>MRKFILSLSILLSALLVACSSRNHYGDTGSLAGLQAMADSKYTRAQKKQKMGKIREMALKETALSVGAQAGLAWRAKIIDEQLNKQARNLDAIYDFNSLVLEHNILPPVLLEGRNTLNLADAQSIRISDRTYKVAKQAHFITTPPTWRQYLWMDYVKPEAPNVTLLPKTKAEKEIWCIYTERGWKNGIDQANTILEENIARIKEDFGGMILYRKLLAMNMVSPPYVSHTDLGVTGDGSEIHIDDRVLRITALPELNVNSAEWRAAVAKDENALERFKNMEKLANQAKIVITNKSWQPIIAPVS[13x];>MNNNKIVIMFIFSALLAGCAGTMKFKKPPINNPSDDATIKLAEAAVSVSDSMLEMAKVEKVITPPSKDNTLTIPNAYNLQARASVDWSGPIEELTARIAKAAHFRFRVLGKSPSVPVLISISTKDESLAEILRDIDYQAGKKASIHVYPNSQVVELRYAKIYS[26x];>[31x]MMAEHDQNNDEYKFAELDSYDMDQAGESDLDSEASYQSGKEGLTKKKDIKRNALIAIGAVVFIMVMYKIIGWMFFSDKSSQVTSKPAIPPVTQVATPQPVQTIPTTTPIQQVQPTTIIEDDPDLKKKVSAIEMTQQSLRSEVNALSEQINAVNNNIKNLNAQIVNLNQIIGNMSNQIARQSEVINVLMARTTPKKVVKVSRPIVQARIIYYIQAVIPGRAWLIGSNGSTLTVREGSKIPGYGMVKLIDSLQGRILTSSGQVIKFSQEDS;>MASKKENLKSLFSNTRTRVIIIFTAALLIIAVVIGFFKIRGATTGSIAAAEVSTVPGGIQSIPGVLDPTAQYAKLQEEQNITQAQVAEKTGGSAIPTIIRTQALGEGVGVIGSQSGVGFAALAQEELGGPQRSLWIQELQDGSCSKSVITKVVNQGAQLTDLKAACSCVQLKDSGYGLQELEQVCECKELKSAGYNARQLKEAGYSAGRLRNCGFDACELRNAGFTAQEMKDGGFSDGELKGAGFSDAEIAKASGLPDGITADDVRKAGCGAAALAKLRQAGVSASAIRKISGCTAEQLKAAGYTAKELKDAGFSAADLRRAGFSAAELKDAGFTARDLLNAGFTPADLAKAGFSDAQIKAAQAELPPGITPQDVKNAGCDVEALKKEREAGVSAALIRQYAGCSAQALKAAGFTDADLANAGFTPAQISAATPLSDAEIKAAGCDPDKLKKLFSAGVSAKRIKELNGCSAEALKAAGYDAQSLLAAGFTPQELLAAGFTPKQLEDAGLNPVSIIADGRVADCSVESLKKARAAGVSALTIKQTLGCSAAALKAAGYTAKELKDAGFTAAELKAAGFSAKELKDAGFTAKELRDAGFSAQELKDVGFSAKDLKDAGFSAAELKAAGFTAAQLKAAGFSAKDLKDAGFSAAELKAAGFSAKELKDAGFSASDLKNAGFSAKELKDAGFSASDLKSAGFSASELKNAGYSADELKKAGYTSAELRNAGFSPQESAVAGLQGPDLQQLDSSITGIPSIPGATPRPTTSDAASSAEQLQAILQKQNEQLAEQKYQQEIQQRTSDMLTAATQLVQDWKQVETQVYTEGTEETKTSGGESAVPGTGTGTGSNNQPVDQGAVSAQNQAIIKTGDIMFAVLDTSVNSDEPGPILATIVTGKLKGSKLIGSFNLPSNADKMVITFNTMSIPGAEKTISISAYAIDPNTARTALASRTNHHYLMRYGSLFASSFLQGFGNAFQSANTTITIGGTGGGNNITVANGVGRSTLENAVIGLATVGKAWSQQAQQLFNTPTTVEVYSGTGLGILFTQDVTTI[18x];>[18x]MMKKYDQLCKYCLVIGLTFSMSCSIYAADQSDDAQQALQQLRMLQQKLSQNPSPDAQSGAGDGGDNAASDSTQQPNQSGQANAPAANQTATAGGDGQIISQDDAEVIDKKAFKDMTRNLYPLNPEQVVKLKQIYETSEYAKAATPGTPPKPTATSQFVNLSPGSTPPVIRLSQGFVSSLVFLDSTGAPWPIAAYDLGDPSSFNIQWDKTSNTLMIQATKLYNYGNLAVRLRGLNTPVMLTLIPGQKAVDYRVDLRVQGYGPNAKSMPTEEGIPPSANDLLLHVLEGVPPPGSRRLVVSGGDARAWLSNEKMYVRTNLTILSPGWLASMTSADGTHAYEMQKSPVLLVSWHGKVMQLKVEGL;>[13x]MRSLRTNYIYVLFKTTGLLFLLLLSACNRSGYIPENEVPKLPCRVDGACDATIIKMMTDLNKKGIKVASVGQNYLISIPASALFADQSPRLNWASYSLLNEIAAFLKQFRKIAITVTSYSSKYVSVKRERALTLARSRVVSEYLWSQGVDSRIIFTQGLGSDKPITSYTLGGDRSPNARVEITFRRAVA;>MRNLMRCLIMIKSLIKGVDMSRKLAKTRILGYGLMICFLAGCFHPPYNNFQPDRRAVKRVGVDTGIGAVAGAIASGTASGTLIGAAAGGTVGLVASIYRDSKRKIIRDLQKQDIQYVEYGDTRTLIIPTDKYFMFSSPRLNEICYPGLNNVIRLLNFYPQSTIYVAGFTDNVGSRSHKRKLSQAQAETMMTFLWANGIAAKRLKAEGYGDKNAISDNAIIHGSAQNRRIEIQWFTSPAQPPQPQMAYVK[13x];>[13x]MLKRCYLLILLMFVLASCAHHKPQTPPAEVKKQGTSSTRQFRQVSSFNQIVVQGRLNVNLHTGYNKPEVMLRGDPRDLVQVRTIVKQNTLYVSLGQGYPDYGAVTVDIKTKFLNRFRYEGAGVVTGNNLRTSYLDLYLANEGTTRLAGNIGLQKLEAVGNGVTQINGVSSRNLQIVLKGDPKVLISGFVNLRQLDMYGKGTLSLYWIKSDTLTIRAKKAAKIQLAGIVNRLDVELWDFAQFKGKYLRAQRSFVKTHDKSVAEISAVNHQSSLATDASDIYYYNLSKTRADFMAFNGSVLDMREWGQSDLKDFDRYNKQFP;>[13x]MLFLKIKTNQRTTMNILKPKAFLLASVFVLSISPAFAADGCCSKMGGINYCDSSAGRLVCNNGFYSTCYCTRHAVMDLQFLMGCCLWHGGVYPQLNSSGLVVCNDGYVSEECSLQK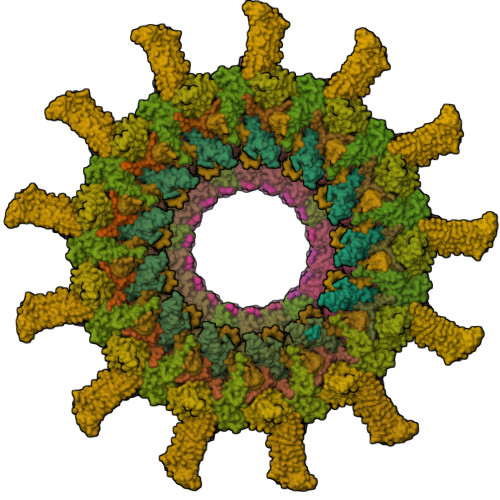PVEQISVY>MSMLQRPGYPNLSVKLFDSYDAWSNNRFVELAATITTLTMRDSLYGRNEGMLQFYDSKNIHTKMDGNEIIQISVANANDINNVKTRIYGCKHFSV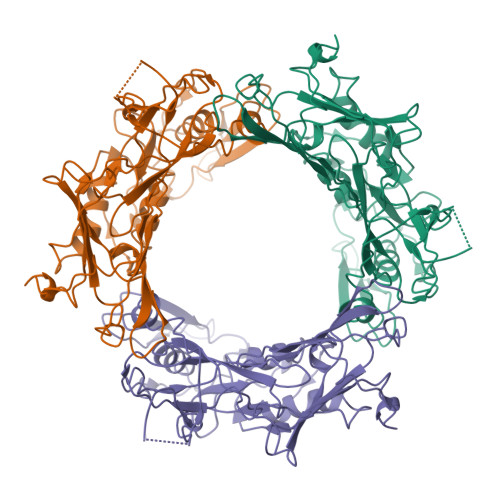SVDSKGDNIIAIELGTIHSIENLKFGRPFFPDAGESIKEMLGVIYQDRTLLTPAINAINAYVPDIPWTSTFENYLSYVREVALAVGSDKFVFVWQDIMGVNMMDYDMMINQEPYPMIVGEPSLIGQFIQELKYPLAYDFVWLTKSNPHKRDPMKNATIYAHSFLDSSIPMITTGKGENSIVVSRSGAYSEMTYRNGYEEAIRLQTMAQYDGYAKCSTIGNFNLTPGVKIIFNDSKNQFKTEFYVDEVIHELSNNNSVTHLYMFTNATKLETIDPVKVKNEFKSDTTTEESSSSNKQ[3x]> GSGSAMGQSTSNHLWLLSDILGQGATANVFRGRHKKTGDLFAIKVFNNISFLRPVDVQMREFEVLKKLNHKNIVKLFAIEEETTTRHKVLIMEFCPCGSLYTVLEEPSNAYGLPESEFLIVLRDVVGGMNHLRENGIVHRDIKPGNIMRVIGEDGQSVYKLTDFGAARELEDDEQFVSLYGTEEYLHPDMYERAVLRKDHQKKYGATVDLWSIGVTFYHAATGSLPFRPFEGPRRNKEVMYKIITGKPSGAISGVQKAENGPIDWSGDMPVSCSLSRGLQVLLTPVLANILEADQEKCWGFDQFFAETSDILHRMVIHVFSLQQMTAHKIYIHSYNTATIFHELV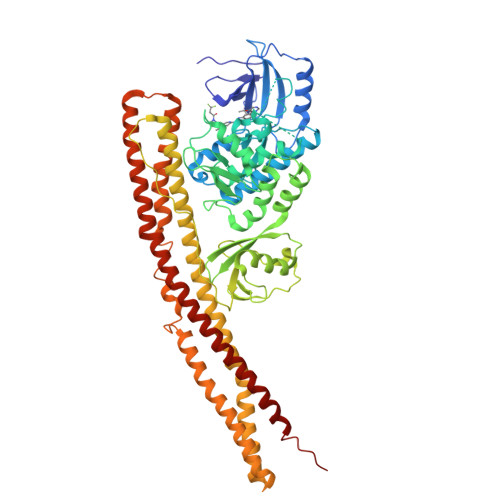YKQTKIISSNQELIYEGRRLVLEPGRLAQHFPKTTEENPIFVVSREPLNTIGLIYEKISLPKVHPRYDLDGDASMAKAITGVVCYACRIASTLLLYQELMRKGIRWLIELIKDDYNETVHKKTEVVITLDFCIRNIEKTVKVYEKLMKINLEAAELGEISDIHTKLLRLSSSQGTIETSLQDIDSRLSPGGSLADAWAHQEGTHPKDRNVEKLQVLLNCMTEIYYQFKKDKAERRLAYNEEQIHKFDKQKLYYHATKAMTHFTDECVKKYEAFLNKSEEWIRKMLHLRKQLLSLTNQCFDIEEEVSKYQEYTNELQET triselane | H2 Se3 | 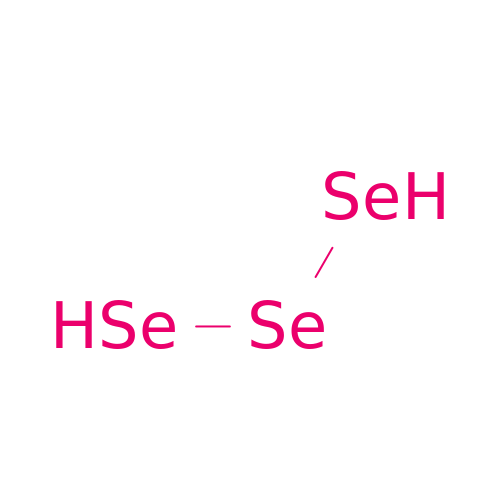GCOIQPYHRLRHMQ-UHFFFAOYSA-N> TIQPGTGYNNGYFYSYWNDGHGGVTYT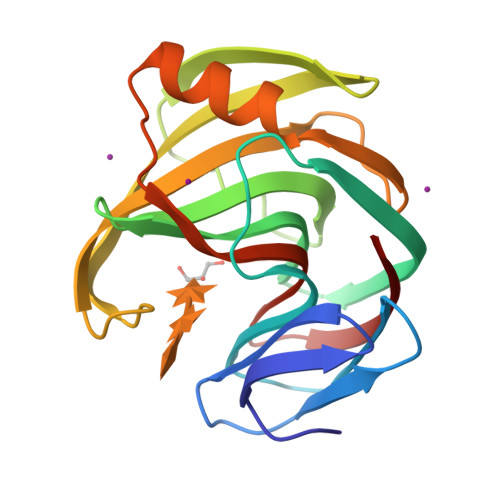NGPGGQFSVNWSNSGNFVGGKGWQPGTKNKVINFSGSYNPNGNSYLSVFGWSRNPLIEYYIVENFGTYNPSTGATKLGEVTSDGSVYDIYRTQRVNQPSIIGTATFYQYWSVRRNHRSSGSVNTANHFNAWAQQGLTLGTMDYQIVAVEGYFSSGSASITVS> MSAEKLFTPLKVGAVTAPNRVFMAPATRLRSIEPGDIPTPLMGEYYRQRASAGLIISEATQISAQAKGYAGAPGLHSPEQIAAWKKITAGVHAEDGRIAVQLWHTGRISHSSIQPGGQAPVSASALNANTRTSLRDENGNAIRVDTTTPRALELDEIPGIVNDFRQAVANAREAGFDLVELHSAHGYLLHQFLSPSSNQRTDQYGGSVENRARLVLEVVDAVCNEWSADRIGIRVSPIGTFQNVDNGPNEEADALYLIEELAKRGIAYLHMSETDLAGGKPYSEAFRQKVRERFHGVIIGAGAYTAEKAEDLIGKGLI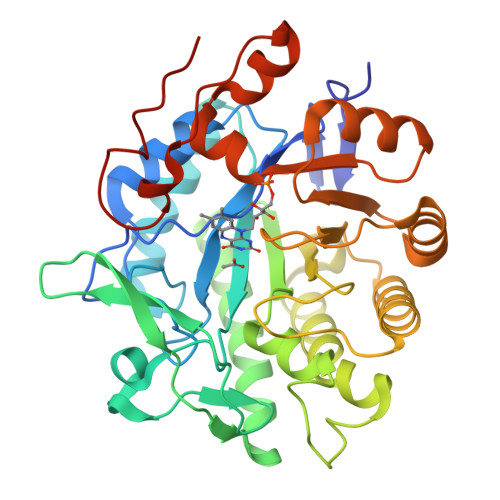DAVAFGRDYIANPDLVARLQKKAELNPQRPESFYGGGAEGYTDYPSLHHHHHHHH>SNAMASLKDVAKLANVSLMTVSRALNTPERLKPETLARVQAAIAETNYVPDLSAKKIRGARATPSTIGVLALDTVTTPFSVEITLSIEETARAHGWNSFVVNMFSDDRPEAVVDLLLSHRPDGIIFTTMGLRQVPLPEKLLTLPCVLANCESLSQPVASYIPDDEQGQYDAVKALLAAGYRRPLCLHLPASQPATIRRRRGLERACREAGIEPDHLSHSYMGQGDEHYHDIPA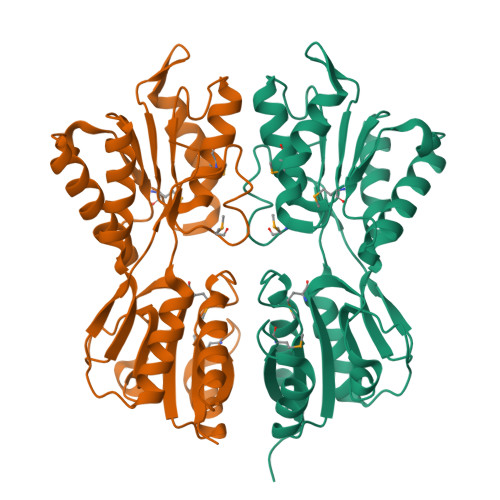VVLAHIREGKPGFDSVICGNDRIAFMVYQTLLGQGLRIPQDVAVVGYDNMVGIGDLFLPPLSTVQLPHYDIGRLSALHIIHGDNHRETRKVASPWLPRASH[2x]>[2x]MNTTPVHALTDIDGGIAVDPAPRLAGPPVFGGPGNDAFDLAPVRSTGREMLRFDFPGVSIGAAHYEEGPTGATVIHIPAGARTAVDARGGAVGLSGGYDFNHAICLAGGAGYGLEAGAGVSGALLERLEHRTGFAELQLVSSAVIYDFSARSTAVYPDKALGRAALEFAVPGEFPQGRAGAGMSASAGKVDWDRTEITGQGAAFRRLGDVRILAVVVPNPVGVIVDRAGTVVRGNYDAQTGVRRHPVFDYQEAFAEQVPPVTEAGNTTISAIVTNVRMSPVELNQFAKQVHSSMHRGIQPFHTDMDGDTLFAVTTDEIDLPTTPGSSRGRLSVNATALGAIASEVMWDAVLEAGK

Nylon hydrolase (NylC) is one of the three enzymes responsible for the endo-type degradation of the by-products of nylon-6 manufacture (cyclic and linear oligomers of 6-aminohexanoate (Ahx) with a degree of polymerization greater than three) and various aliphatic nylons (e.g., nylon-6 and nylon-66). However, the post-translational autocleavage of the nascent polypeptide between Asn266 and Thr267 generates an active enzyme with an α subunit (27 kDa) and a β subunit (9 kDa). Based on the X-ray-crystallographic structure of NylCA, we reported that four αβ heterodimers (molecules A-D) form a doughnut-shaped quaternary structure. In addition, we proposed that the nucleophilic N-terminal residue Thr267 in the β subunit functions as a catalytic residue for either autocleavage (from precursor to active enzyme) or substrate hydrolysis.

Among the various mutants obtained from wild-type NylCp2, which differ in thermostability, a single D122G mutation drastically improves the thermostability by 24 °C9. However, the D2 symmetry was partly altered by mutations at position 122. Plotting the protein stability (Tm value) estimated from the CD analyses against the distance between the two monomer molecules revealed that the protein stability exhibited an inverse correlation with the a2/a1 ratio (index of symmetry). In other words, the ratio changed from 0.979 to 1.197 from the wild-type (Asp122) to the mutant (Arg122, Lys122, Val122, and Gly122) enzyme, although this value should be equal to one for a perfectly symmetric structure. In wild-type NylCp2, Lys159-NH3+ (located on helix α2 in molecule A) was 2.87 Å away from Glu115-Oε1− (located on helix α1 in molecule D). In contrast, the distance was reduced to 2.65 Å in the thermostable Gly122 enzyme. Notably, this distance decreased with an almost linear correlation with increasing thermostability in the wild-type and mutant enzymes. We suggest that the electrostatic effect between the two residues will enhance the subunit binding around Gly122 of helix α1.> AMAISNWVNVISDLKKIEDLIQSMHIDATLYTESDVHP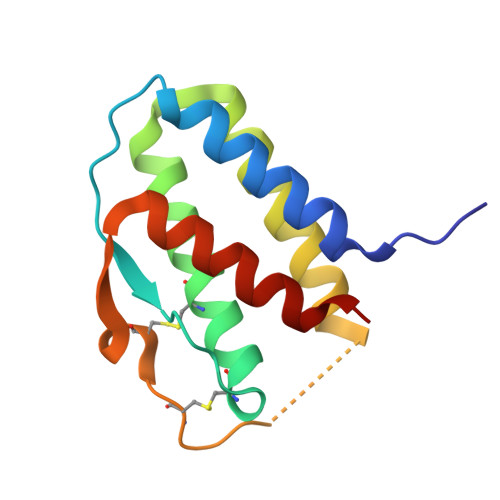SCKVTAMKCFLLELQVISLESGDASIHDTVENLIILANNSLSSNGNVTESGCKECEELEEKNIKEFLQSFVHIVQMFINTS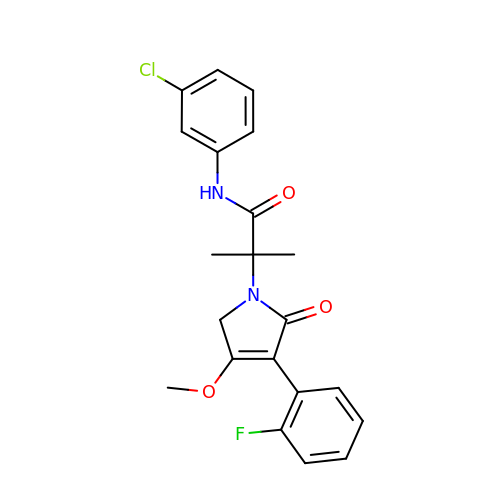~{N}-(3-chlorophenyl)-2-[4-(2-fluorophenyl)-3-methoxy-5-oxidanylidene-2~{H}-pyrrol-1-yl]-2-methyl-propanamide | C21 H20 Cl F N2 O3 | NSSJIPGWTMBBIM-UHFFFAOYSA-N>[6x]MIQQTGYSKKVMEHFMNPRNVGVIDDPDGYGKVGNPVCGDLMEIFIKVGDEKIEDIKFRTFGCGAAIATSSMITEMARGKSLEEAMRITRNDVADALDGLPPQKMCCSNLAADALHAAIN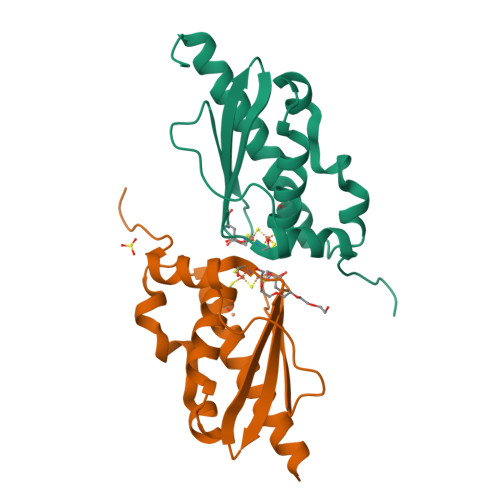DYLSKKQKHLEH> GSPPAQLSVHTVSWNSGHERAPTNLEELLGLNSGETPDVIAVAVQGFGFQTDKPQQGPACVKNFQSLLTSKGYTKLKNTITETMGLTVYCLEKHLDQNTLKNETIIVTVDDQKKSGGIVTSFTIYNKRFSFTTSRMSDEDVTSTNTKYAYDTRLDYSKKDDPSDFLFWIGDLNVRVETNATHAKSLVDQNNIDGLMAFDQLKKAKEQKLFDGWTEPQVTFKPTYKFKPNTDEYDLSATPSWTDRALYKSGTGKTIQPLSYNSLTNYKQTEHRPVLAKFRV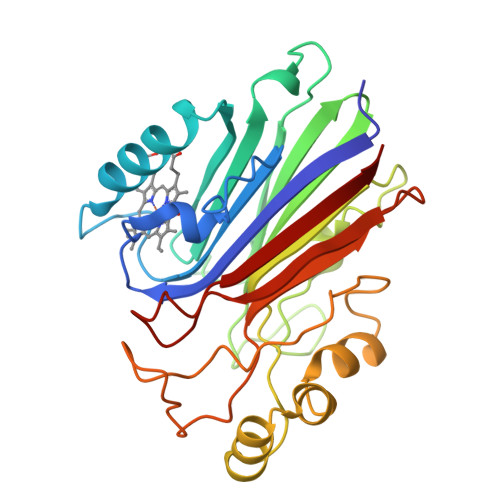TL>[2x]AETTPWGQTFVGATVLSDSQAGNRTICIIDSGYDRSHNDLNANNVTGTNNSGTGNWYQPGNNNAHGTHVAGTIAAIANNEGVVGVMPNQNANIHIVKVFNEAGWGYSSSLVAAIDTCVNSGGANVVTMSLGGSGSTTTERNALNTHYNNGVLLIAAAGNAGDSSYSYPASYDSVMSVAAVDSNLDHAAFSQYTDQ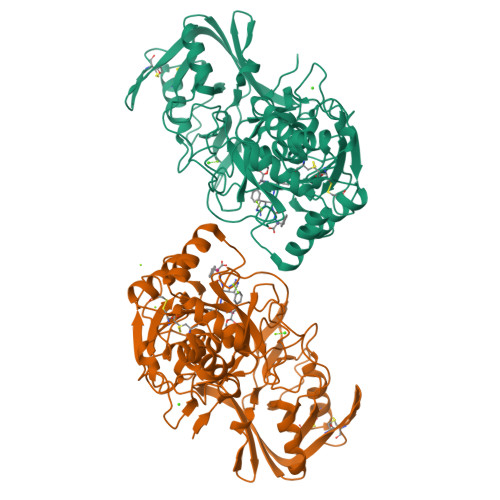VEISGPGEAILSTVTVGEGRLADITIGGQSYFSNGVVPHNRLTPSGTSYAPAPINASATGALAECTVNGTSFSCGNMANKICLVERVGNQGSSYPEINSTKACKTAGAKGIIVYSNSALPGLQNPFLVDANSDITVPSVSVDRATGLALKAKLGQSTTVSNQGNQDYEYYNGTSMATPHVSGVATLVWSYHPECSASQVRAALNATADDLSVAGRDNQTGYGMINAVAAKAYLDESCTGPTDPGTG> MAERQEEQRGSPPLRAEGKADAEVKLILYHWTHSFSSQKVRLVIAEKALKCEEHDVSLPLSEHNEPWFMRLNSTGEVPVLIHGENIICEATQIIDYLEQTFLDERTPRLMPDKESMYYPQVQHYRELLDSLPMDAYTHGCILHPELTVDSMIPAYATTRIRSQIGNTESELKKLAEENPDLQEAYIAKQKRLKSKLLDHDNVKYLKKILDELEKVLDQVETELQRRNEETPEEGQQPWLCGESFTLADVSLAVTLHRLKFLGFARRNWGNGKRPNLETYYERVLKRKTFNKVLGHVNNILIS

The ganglioside-induced differentiation-associated protein 1 (GDAP1) is an integral MOM protein, proposed to have an auxiliary role in mitochondrial fission and fusion, possibly via redox-dependent interactions with cytoskeletal components. GDAP1 has two GST-like domains, followed by a transmembrane helix, which anchors the protein into the MOM. Structural data have shown a covalently bound dimer interface in GDAP1, and while dimerisation is a common feature in catalytic GSTs, the GDAP1 dimer is formed differently, with a unique interface having a central disulphide bridge between Cys88 from each subunit. We carried out structural and biophysical analyses on several CMT-linked GDAP1 protein variants and describe new crystal structures of the autosomal recessive R120Q and the autosomal dominant A247V and R282H GDAP1 variants.

The R120Q mutation is located close to the N-terminal end of the α3 helix. Due to the mutation, residue 120 loses contact with the α6-α7 loop tip at Cys240, whereby the hydrogen bond between the Arg120 side chain and the backbone carbonyl of Cys240 is lost. This is further linked to alterations in surrounding side chain conformations. Arg120 participates in a hydrogen bond network between helices α3 and α6. Arg120 in GDAP1 is a target of several CMT mutations, and its interactions with the backbone carbonyl of Cys240 in the ⍺6-⍺7 loop appear central. Structures of the mutants R120Q and R120W indicate loosening of the structure locally, as well as loss of the hydrogen bond, which is accompanied by a decrease in observed heat stability in R120Q and R120W. Arg120 is not conserved in GSTs at the sequence level; however, an Arg residue from the neighbouring helix in GST reaches the same position and makes similar interactions to the same carbonyl group in the ⍺6-⍺7 loop. In essence, all substitutions to Arg120 are unfavourable; this shows that the interactions made by Arg120 are important for folding and stability. This is in line with our experimental data for both R120Q and R120W, which indicate minor changes in structure, but destabilisation of the fold. Also R120Q had a slightly different conformation, most clearly seen in the distance distribution.>[2x]MDVSFEFEHYQVRLIKSSDAVTIANYFMRNRHHLAPWEPKRSHAFFTPEG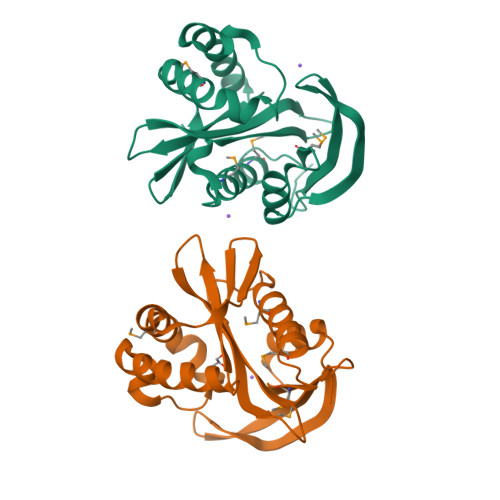WKQRLLQLVELHKHNLAFYFVVVDKNEHKIIGTVSYSNITRFPFHAGHVGYSLDSEYQGKGIMRRAVNVTIDWMFKAQNLHRIMAAYIPRNEKSAKVLAALGFVKEGEAKKYLYINGAWEDHILTSKINDDWKP>MTRQMILAVGQQGPIARAETREQVVGRLLDMLTNAASRGVNFIVFPELALTTFFPRWHFTDEAELDSFYETEMPGPVVRPLFETAAELGIGFNLGYAELVVEGGVKRRFNTSILVDKSGKIVGKYRKIHLPGHKEYEAYRPFQHLEKRYFEPGDLGFPVYDVDAAKMGMFICNDRRWPETWRVMGLKGAEIICGGYNTPTHNPPVPQHDHLTSFHHLL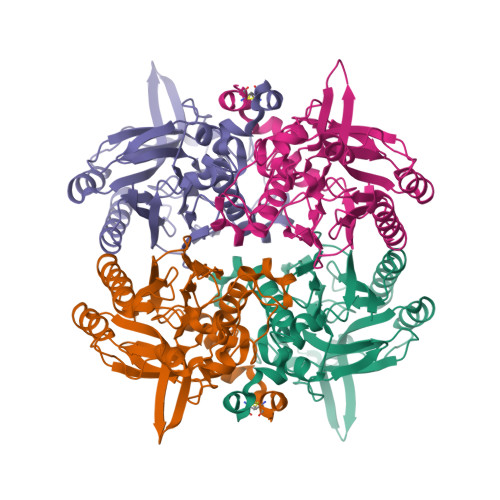SMQAGSYQNGAWSAAAGKVGMEEGCMLLGHSCIVAPTGEIVALTTTLEDEVITAALDLDRCRELREHIFNFKAHRQPQHYGLICEF[4x]> MQASQFSAQVLDWYDKYGRATLPW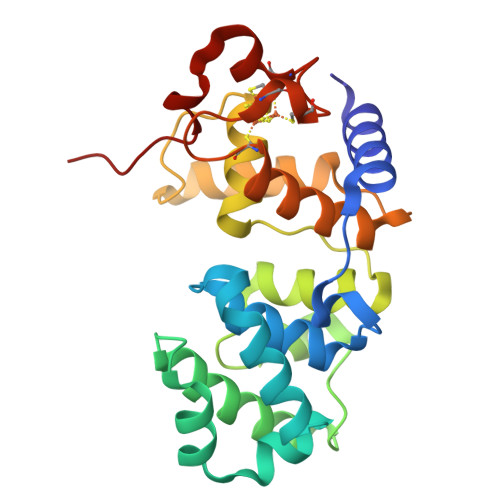QIDKTPYKVWLSEVMLQQTQVATVIPYFERFMARFPTVTDLANAPLDEVLHLWTGLGYYARARNLHKAAQQVATLHGGKFPETFEEVAALPGVGRSTAGAILSLSLGKHFPILDGNVKRVLARCYAVSGWPGKKEVENKLWSLSEQVTPAVGVERFNQAMMDLGAMICTRSKPKCSLCPLQNGCIAAANNSWALYPGKKPK> MKHHHHHHHGAAGTSLYKKAGENLYFQGSMKADYKKINSILTYTSTALKNPKIIKDKDLVVLLTIIQEEAKQNRIFYDYKRKFRPAVTRFTIDNNFEIPDCLVKL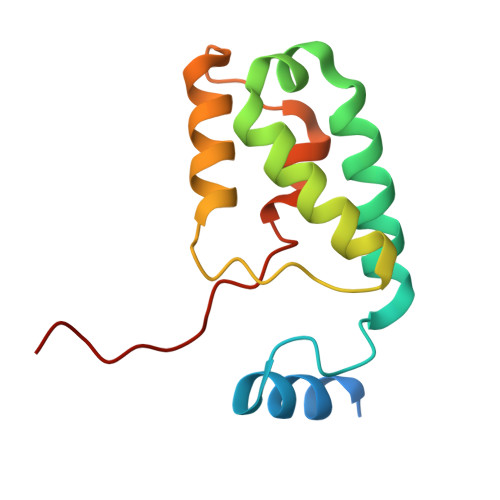LSAVETPKAWSGFS> DVGDEYEIIETIGNGAYGVVSSARRRLTGQQVAIKKIPNAFDVVTNAKRTLRELKILKHFKHDNIIAIKDILRPTVPYGEFKSVYVVLDLMESDLHQIIHSSQPLTLEHVRYFLYQLLRGLKYMHSAQVIHRDLKPSNLLVNENCELKIGDFGMARGLCTSPAEHQYFMTEYVATRWYRAPELMLSLHEYTQAIDLWSVGCIFGEMLARRQLFPGKNYVHQLQLIMMVLGTPSPAVIQAVGAERVRAYIQSLPPRQPVPWETVYPGADRQALSLLGRMLRFEPSARISAAAALRHPFLAKYHDPDDEPDCAPPFDFAFDREALTRERIKEAIVAEIEDFHARRE

The ERK5 protein, which is encoded by the MAPK7 gene, comprises an N-terminal kinase domain and a large C-terminal domain containing transcriptional transactivating functionality and nuclear localization and export sequences (NLS/NES). ERK5 is the effector kinase of a canonical kinase module comprising MEK (MAPK/ERK kinase) 5, MEKK (MEK kinase) 2/3 and ERK5 itself.

Compounds 2 and 3, like compound 1, bind at the conventional ATP-binding site, while compounds 4, 5 and 6 bind at a novel allosteric binding site. The allosteric binding site is a cryptic site that is absent from other structures of ERK5 and is located between the P-loop and the αC helix. The so-called gatekeeper residue Leu137 lies within 3.5 Å of the methyl substituent on the phenyl ring of compound 5. As a consequence of the binding of compounds 4–6, the P-loop is pushed away from the αC helix towards the ATP-binding site, suggesting that these allosteric inhibitors will also be ATP-competitive. An ATP-competition study was therefore carried out to verify this hypothesis. A comparison of the IC50 curves at different ATP concentrations for the allosteric inhibitor 5 and the reference compound 2 shows that with increasing ATP concentration the IC50 values for both compounds 2 and 5 consistently increase. Kinase-selectivity screening showed compound 5 to be more selective than the type I inhibitors 2 and 3, with significant activity against only five kinases out of the 225 tested. Consistent with the differences in amino-acid composition of the allosteric binding pocket, compound 5 showed less than 10% inhibition when tested against a panel of MAP kinases including ERK1, ERK2 and p38.>MASKQNDKDGAVRRDASFECGVKAGDWLPGFTPREETVYVHGGVEPDPLTGAILPPIYQNTTFVQESVENYLSKGFSYSRTSNPTVLSLEKKIAEIEGGFGACCFATGMAATVTIFSAFLAPGDHCLVTNCSYGGTNRCARLHFSKYNIDFEFIDFRDPTNVEKAIRPQTKVVFSESPCNPTLYLADIEAISQICKEKKVLHVCDSTFATPYMMRPLDLGADIVVQSTTKYYDGHNCTLGGAVISSTKEIHDKVFFLRNVMGNIMSAQTAFYTLLTLKTLPIRVEKQSANAQKIAEFLSKHHKVEHVIYPGIPSFPQKELALKQHKNVHGGMLAFEVKGGTEAGIRMMNHVPR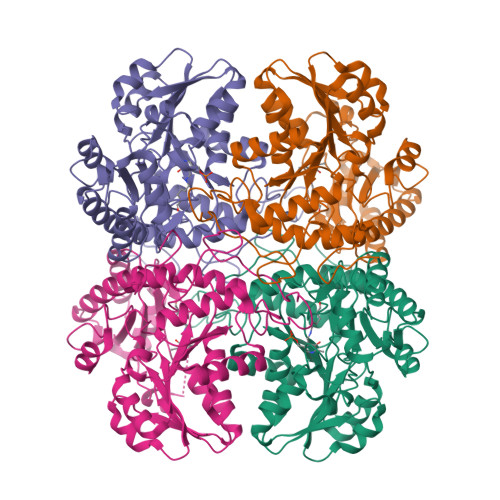PWSLCENLGACESIITCPAVFTHANMLREDRLKVGITDGFIRVSVGIEDVNDLIDGLDYALSKA[8x]>[6x]MYKHTIVYDGEVDKISATVVGWGYNDGKILICDIKDYVPGQTQNLYVVGGGACEKISSITKEKFIMIKGNDRFDTLYKALDFINR

Endolysins are produced by many double stranded DNA bacteriophages to effect the release of new virions from an infected cell by degrading the bacterial cell wall. Endolysins typically consist of a peptidoglycan hydrolase domain and a C-terminal domain that is often termed as a cell wall binding domain. Here, we present the crystal structures of autoproteolytic fragments of the CD27L and CTP1L endolysins, covering the C-terminal domain. We propose that the cleavage and oligomerization are linked, and they provide the endolysin with a trigger and release mechanism that leads to activation.

When crystallization trials for full length CD27L endolysin were set up, crystals appeared overnight from freshly purified protein. An X-ray data set to 2.3 Ångstrom was collected from a fresh crystal, and it was realized that the crystal most likely contained the C-terminal portion of the endolysin, because molecular replacement with the previously determined crystal structure of the catalytic domain was not successful. The structure was used as a model to solve the structure of the full-length CD27L crystals by molecular replacement. It was found that the “full length” construct had been proteolyzed and the crystal contained six copies of the C-terminal portion of CD27L alone. The refined structure shows clear electron density for all six monomers of the C-terminal domain with a Matthews coefficient of 2.3, and there is no space in the crystal lattice for an additional N-terminal domain. The C-terminal portion of CD27L consists of a platform of four parallel beta strands, flanked by an alpha helix with two additional alpha helices mounted on top. The autolytic fragment of the C-terminal domain starts at the end of the linker at methionine M186, which is still integrated in the C-terminal domain. The proteolytic fragments of CD27L form a mixture of dimers within the crystal lattice. All six molecules are engaged in one common dimerization mode, where the alpha helices α1 and α3 from one molecule stack on their symmetry mate from a second molecule. The dimerization is such that the N-termini of both monomers are pointing away from the dimer interface, and we term this dimerization mode a ‘head-on’ dimer. An alternative dimerization mode is found among the six C-terminal domains present in the crystal structure of the proteolytic fragment of CD27L endolysin, between two molecules that are each involved in separate head-on dimers as well.>MSLTSPKRNIVGFTIVNDKHEFAQRLINAFKAEAKANKYEALVATSQNSRISEREQILEFVHLKVDAIFITTLDDVYIGSAIEEAKKAGIPVFAIDRMIRSDAVVSSITSNNQMIGEQLASYIKNELIKQTGRSTGRIVEITGTANVYTTNERHRGFLKGIENEPTLSIVDSVSGNYDPVTSERVMRQVI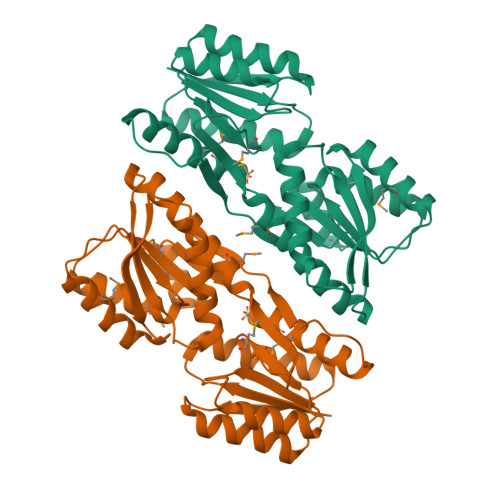DSGIPFDAVYCHNDDIAMGVLEALKKAKISGKIVVGIDGNRAILEAVDMKSMDATVVQSAEEMMKVAFSALKLHTKNKKIPDRFYTYSYLYDGSREGHHHHHH[2x]> EPTAEMLTNNCAGCHGTHGNSVGPASPSIAQMDPMVFVEVMEGFKSGEI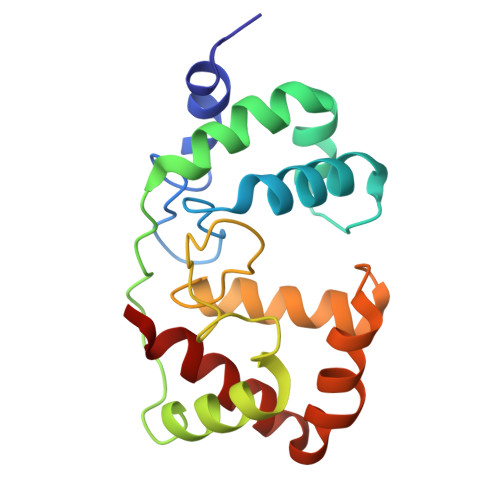ASTIMGRIAKGYSTADFEKMAGYFKQQTYQPAKQSFDTALADTGAKLHDKYCEKCHVEGGKPLADEEDYHILAGQWTPYLQYAMSDFREERRPMEKKMASKLRELLKAEGDAGLDALFAFYASQQ> GIDPFTQNGYENPTYKF;> PVQLNLLYVQARDDILNGSHPVSFDKACEFAGYQCQIQFGPHNEQKHKPGFLELKDFLPKEYIKQKGERKIFMAHKNCGNMSEIEAKVRYVKLARSLKTYGVSFFLVKEKMK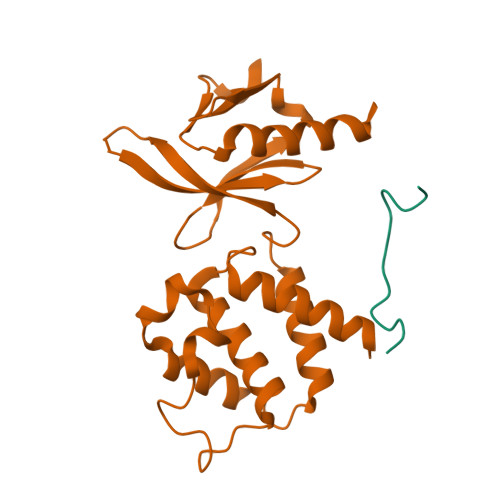GKNKLVPRLLGITKECVMRVDEKTKEVIQEWSLTNIKRWAASPKSFTLDFGDYQDGYYSVQTTEGEQIAQLIAGYIDIIL> QDNSRYTH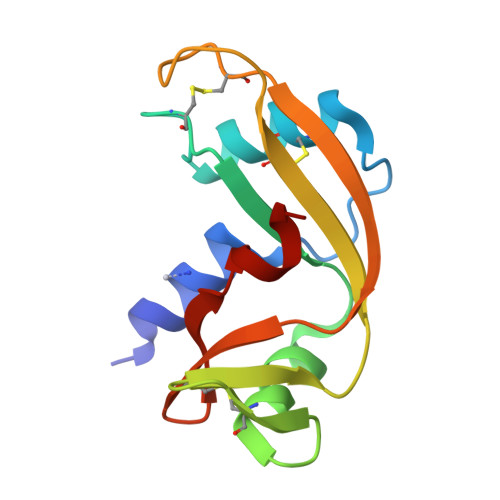FLTQHYDAKPQGRDDRYCESIMRRRGLTSPCKDINTFIHGNKRSIKAICENKNGNPHRENLRISKSSFQVTTCKLHGGSPWPPCQYRATAGFRNVVVACENGLPVHLDQSIFRRP>[5x]LDRADILYNIRQTSRPDVIPTQRDRPVAVSVSLKFINILEVNEITNEVDVVFWQQTTWSDRTLAWNSSHSPDQVSVPISSLWVPDLAAYNAISKPE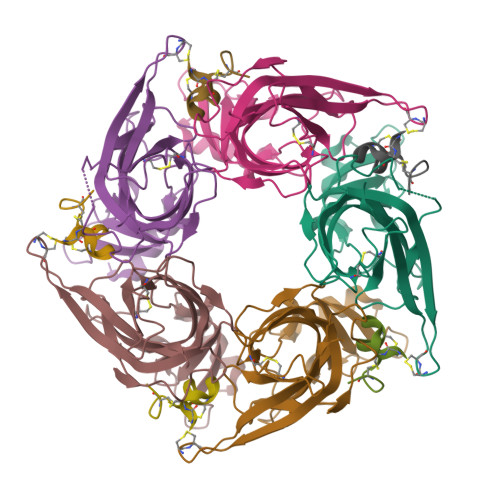VLTPQLARVVSDGEVLYMPSIRQRFSCDVSGVDTESGATCRIKIGSWTHHSREISVDPTTENSDDSEYFSQYSRFEILDVTQKKNSVTYSCCPEAYEDVEVSLNFRKKGRSEIL;>GCCSHPACNVNNPHICGX[5x]> GSHMM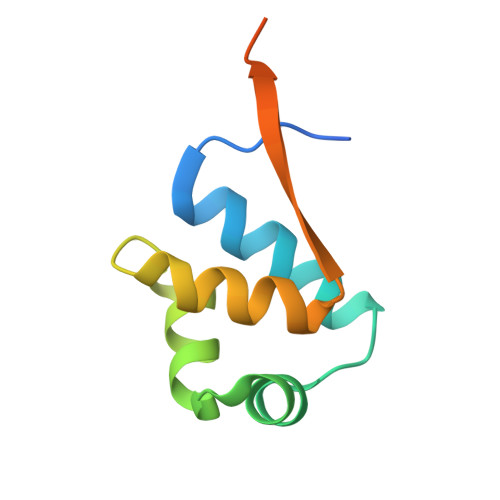SFQKIYSPTQLANAMKLVRQQNGWTQSELAKKIGIKQATISNFENNPDNTTLTTFFKILQSLELSMTLCDTKNASPESTEQQDLEW> SAKDE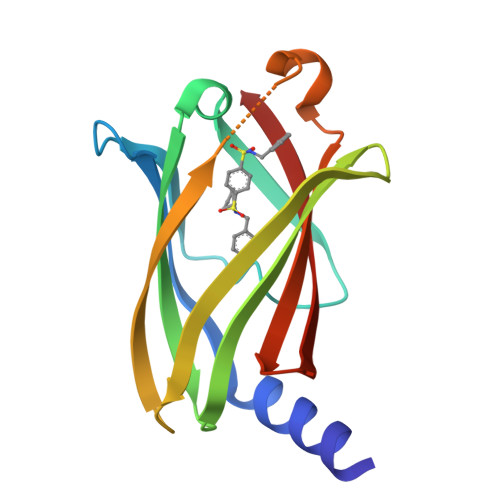RAREILRGFKLNWMNLRDAETGKILWQGTEDLSVPGVEHEARVPKKILKCKAVSRELNFSSTEQMEKFRLEQKVYFKGQCLEEWFFEFGFVIPNSTNTWQSLIEAAPESQMMPASVLTGNVIIETKFFDDDLLVSTSRVRLFYV>MSLDKVMVVAEVRPSEDVNKVLSAISNFFDFEKMNTRKEGIIDILVLEARTLKSLLKFHRVLRNERILDSARKYLMKGIEGNTIAFMIHKQAAAVGVLSFVDSDKESPLGAIKFYIEYQNPKEIVDWLAPKTAHGVPLWDNPVPPDVEGHHHHHH[2x]

UPF0201 family proteins constitute one such uncharacterized, archaeal specific protein family. The UPF0201 family proteins occur as a single globular α/β domain with approximate dimensions of 55×35×35 Å3. The protomeric structure consists of a five-stranded, anti-parallel β-sheet, five α helices, which are located on one face of the β-sheet, and three loops connecting helices and strands. We have further documented that all members of this archaeal specific protein family share a common polypeptide chain fold, which is evolutionarily related to the RRM motif found in the ribosomal L5 proteins and many other RNA-binding proteins.

For 10077b and 10077c from S. solfataricus and S. solfataricus P2, respectively, full-length constructs bearing C-terminal His6 tags yielded crystals and structures. In none of the three X-ray structures of full-length UPF0201 proteins was electron density corresponding to the 15–20 C-terminal residues observed. The loop connecting β2 and β3 protrudes somewhat from the globular domain, and the electron density corresponding to this region is poorly defined in the 10077b and 10077d structures. The polypeptide chains of 10077a and 10077b extend beyond the C-terminal helix, α5, for about 20 residues, and form a type IV turn followed by random coil. Pairwise sequence identities among the structures we report herein range between 15–22%, with exception of 10077a and 10077b, which are 35% identical. Our four UPF0201 structures represent subfamilies N149845 (10077a, b) and N130963 (10077c, d). The crystallographic asymmetric units contain one protomer in 10077c, two in 10077b and four protomers in both 10077a and 10077d. While 10077a, 10077b and 10077d all form one type of dimer (typeI), 10077c forms altogether different dimer via crystallographic symmetry (typeII). The interface surface area for type I dimers in 10077a, 10077b and 10077d are 672, 563 and 611 Å2, respectively.>GSHMNQPSSLAADLRGAWHAQAQSHPLITLGLAASAAGVVLLLVAGIVNALTGENRVHVGYAVLGGAAGFAATALGALMALGLRAISARTQDAMLGFAAGMMLAASAFSLILPGLDAAGTIVGPGPAAAAVVALGLGLGVLLMLGLDYFTPHEHERTGHQGPEAARVNRVWLFVLTIILHNLPEGMAIGVSFATGDLRIGLPLTSAIAIQDVPEGLAVALALRAVGLPIGRAVLVAVASGLMEPLGALVGVGISSGFALAYPISMGLAAGAMIFVVSHEVIPETHRNGHETTATVGLMAGFALMMFLDTALG[2x]

Due to their key role in Zn2+ homeostasis, ZIP transporters are broadly represented in animals, plants, protozoans, prokaryotes, and archaea. In bacteria, there are two main zinc uptake transporters, the ZnuABC transporter and the ZIP family transporter. ZupT proteins are members of the ZIP family. Bacterial ZIPs do not have a large intracellular domain, but contain a histidine-rich loop between TM3-4.

In this work, we determined a dimer structure of BbZIP in an inward-facing, inhibited conformation. To overcome the non-outer membrane issue, we reconstituted purified BbZIP into the small amphipol PMAL-C8 to form BbZIP-PMAL-C8 nanoparticles. The final refined dimer reconstruction contains 37,954 particles at a resolution of 3.05 Å as estimated by the gold standard Fourier Shell Correlation (FSC) at 0.143. The dimer structure consists of 18 transmembrane helices, nine from each protomer. Cd2+ has been shown to help stabilize the protein for crystallization, so we used Cd2+ in our protein purification and found six Cd2+ ions in the dimer. In each monomer, two Cd2+ ions are in the M1 and M2 binuclear sites in the middle of TM2, TM4, and TM5 as previously reported in the crystal structure. The third ion binds to a site (M3) near the cytoplasmic surface that consists of residues Asp144 on TM3, Glu276 on TM7, and two histidine residues, His149 and His151, on a loop (residues 146–166) between TM3 and TM4. The cryo-EM density for the M1-site Cd2+ is much higher than the M2-site Cd2+, indicating a partial occupancy in the M2 site. His149 and His151 are on the loop L(3,4) which is disordered in the crystal structure but is well ordered in the cryo-EM structure through the formation of the M3 site. Two modeled PE molecules interact with both monomers and might contribute to the stabilization of the dimer.(1R,9S)-13-(3,5-dimethoxy-4-oxidanyl-phenyl)carbonyl-11,13-diazatricyclo[7.3.1.0^{2,7}]trideca-2,4,6-trien-10-one 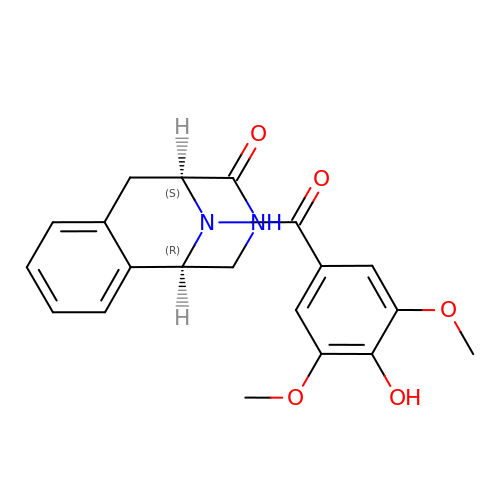| C20 H20 N2 O5 | JRZNNUGTWNEAQO-GJZGRUSLSA-N> GDQQEPYYGNSEVKMPQIDSEWNLELMPNRSGQYWKVFVYKDLKYNALFTRSLGWNGGDGVFTTGLPDGNIFWSFNDSFYGVINENRSRGNCSFPRNSIMVQTPGEKDENLVWLADYVQTNDPNADRYYQVRTHIRHPKATLSDEKIQAGEIDQDYLYWAGDATIYNNQMQMLWGAVDNTDPNNLMRRFGTCLATYSLEGKPGDATYMKLISRNDNFNDHTLGYGDTMWEDEDGHIYLYTTSNYKVAVARTATRDLGSQWE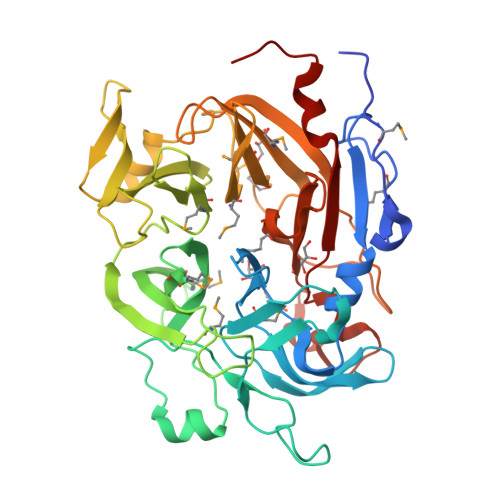YYVADPQGHFSWTTQYPSTQDAENSTIIPLESACSMPWVFKKGDTYYMIGQSMWFGRDVLMFRSKHPYGPFVDQKTLFTLPEFLDKIGEQRYQHVYMVNIHPALSRTGELVISTNTDCSNFWDNFNAPGSADFYRPYFYRVFNWESLYDNDAPLE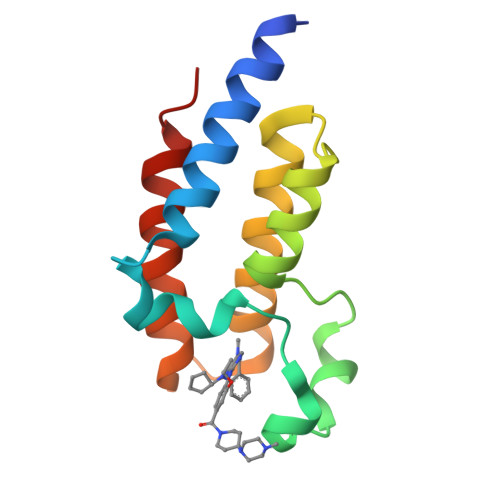>[4x]GAASTVKVTEQLRHCSEILKEMLAKKHFSYAWPFYNPVDVNALGLHNYYDVVKNPMDLGTIKEKMDNQEYKDAYKFAADVRLMFMNCYKYNPPDHEVVTMARMLQDVFETHFSKIPI> MSDNRRRRREEDDSDSENELPPSSPQQHFRGGMNPVSSPIGSPDMINPEGDDNEVDDVPDIDEVEEQMNEVDLMDDNMYEDYAADHNRDRYDPDQVDDREQQELSLSERRRIDAQLNERDRLLRNVAYIDDEDEEQEGAAQLDEMGLPVQRRRRRRQYEDLENSDDDLLSDMDIDPLREELTLESLSNVKANSYSEWITQPNVSRTIARELKSFLLEYTDETGRSVYGARIRTLGEMNSESLEVNYRHLAESKAILALFLAKCPEEMLKIFDLVAMEATELHYPDYARIHSEIHVRISDFPTIYSLRELRESNLSSLVRVTGVVTRRTGVFPQLKYVKFNCLKCGSILGPFFQDSNEEIRISFCTNCKSKGPFRVNGEKTVYRNYQRVTLQEAPGTVPPGRLPRHREVILLADLVDVSKPGEEVEVTGIYKNNYDGNLNAKNGFPVFATIIEANSIKRREGNTANEGEEGLDVFSWTEEEEREFRKISRDRGIIDKIISSMAPSIYGHRDIKTAVACSLFGGVPKNVNGKHSIRGDINVLLLGDPGTAKSQILKYVEKTAHRAVFATGQGASAVGLTASVRKDPITKEWTLEGGALVLADKGVCLIDEFDKMNDQDRTSIHEAMEQQSISISKAGIVTTLQARCSIIAAANPNGGRYNSTLPLAQNVSLTEPILSRFDILCVVRDLVDEEADERLATFVVDSHVRSHPENDEDREGEELKNNGESAIEQGEDEINEQLNARQRRLQRQRKKEEEISPIPQELLMKYIHYARTKIYPKLHQMDMDKVSRVYADLRRESISTGSFPITVRHLESILRIAESFAKMRLSEFVSSYDLDRAIKVVVDSFVDAQKVSVRRQLRRSFAIYTLGH;> MEGSTGFDGDATTFFAPDAVFGDRVRRFQEFLDTFTSYRDSVRSIQVYNSNNAANYNDDQDDADERDLLGDDDGDDLEKEKKAASSTSLNILPHRIIISLDDLREFDRSFWSGILVEPAYFIPPAEKALTDLADSMDDVPHPNASAVSSRHPWKLSFKGSFGAHALSPRTLTAQHLNKLVSVEGIVTKTSLVRPKLIRSVHYAAKTGRFHYRDYTDATTTLTTRIPTPAIYPTEDTEGNKLTTEYGYSTFIDHQRITVQEMPEMAPAGQLPRSIDVILDDDLVDKTKPGDRVNVVGVFKSLGAGGMNQSNSNTLIGFKTLILGNTVYPLHARSTGVAARQMLTDFDIRNINKLSKKKDIFDILSQSLAPSIYGHDHIKKAILLMLMGGVEKNLENGSHLRGDINILMVGDPSTAKSQLLRFVLNTASLAIATTGRGSSGVGLTAAVTTDRETGERRLEAGAMVLADRGVVCIDEFDKMTDVDRVAIHEVMEQQTVTIAKAGIHTTLNARCSVIAAANPVFGQYDVNRDPHQNIALPDSLLSRFDLLFVVTDDINEIRDRSISEHVLRTHRYLPPGYLEGEPVRERLNLSLAVGEDADINPEEHSNSGAGVENEGEDDEDHVFEKFNPLLQAGAKLAKNKGNYNGTEIPKLVTIPFLRKYVQYAKERVIPQLTQEAINVIVKNYTDLRNDDNTKKSPITARTLETLIRLATAHAKVRLSKTVNKVDAKVAANLLRFALLGEDIGNDIDEEESEYEEALSKRSPQKSPKKRQRVRQPASNSGSPIKSTPRRSTASSVNATPSSARRILRFQDDEQNAGEDDNDIMSPLPADEEAELQRRLQLGLRVSPRRREHLHAPEEGSSGPLTEVGTPRLPNVSSAGQDDEQQQSVISFDNVEPGTISTGRLSLISGIIARLMQTEIFEEESYPVASLFERINEELPEEEKFSAQEYLAGLKIMSDRNNLMVADDKVWRV;> MSQQSSSPTKEDNNSSSPVVPNPDSVPPQLSSPALFYSSSSSQGDIYGRNNSQNLSQGEGNIRAAIGSSPLNFPSSSQRQNSDVFQSQGRQGRIRSSASASGRSRYHSDLRSDRALPTSSSSLGRNGQNRVHMRRNDIHTSDLSSPRRIVDFDTRSGVNTLDTSSSSAPPSEASEPLRIIWGTNVSIQECTTNFRNFLMSFKYKFRKILDEREEFINNTTDEELYYIKQLNEMRELGTSNLNLDARNLLAYKQTEDLYHQLLNYPQEVISIMDQTIKDCMVSLIVDNNLDYDLDEIETKFYKVRPYNVGSCKGMRELNPNDIDKLINLKGLVLRSTPVIPDMKVAFFKCNVCDHTMAVEIDRGVIQEPARCERIDCNEPNSMSLIHNRCSFADKQVIKLQETPDFVPDGQTPHSISLCVYDELVDSCRAGDRIEVTGTFRSIPIRANSRQRVLKSLYKTYVDVVHVKKVSDKRLDVDTSTIEQELMQNKVDHNEVEEVRQITDQDLAKIREVAAREDLYSLLARSIAPSIYELEDVKKGILLQLFGGTNKTFTKGGRYRGDINILLCGDPSTSKSQILQYVHKITPRGVYTSGKGSSAVGLTAYITRDVDTKQLVLESGALVLSDGGVCCIDEFDKMSDSTRSVLHEVMEQQTISIAKAGIITTLNARSSILASANPIGSRYNPNLPVTENIDLPPPLLSRFDLVYLVLDKVDEKNDRELAKHLTNLYLEDKPEHISQDDVLPVEFLTMYISYAKEHIHPIITEAAKTELVRAYVGMRKMGDDSRSDEKRITATTRQLESMIRLAEAHAKMKLKNVVELEDVQEAVRLIRSAIKDYATDPKTGKIDMNLVQTGKSVIQRKLQEDLSREIMNVLKDQASDSMSFNELIKQINEHSQDRVESSDIQEALSRLQQEDKVIVLGEGVRRSVRLNNRV;> MSFDRPEIYSAPVLQGESPNDDDNTEIIKSFKNFILEFRLDSQFIYRDQLRNNILVKNYSLTVNMEHLIGYNEDIYKKLSDEPSDIIPLFETAITQVAKRISILSRAQSANNNDKDPENTSMDTDSLLLNSLPTFQLILNSNANQIPLRDLDSEHVSKIVRLSGIIISTSVLSSRATYLSIMCRNCRHTTSITINNFNSITGNTVSLPRSCLSTIESESSMANESNIGDESTKKNCGPDPYIIIHESSKFIDQQFLKLQEIPELVPVGEMPRNLTMTCDRYLTNKVIPGTRVTIVGIYSIYNSKNGAGSGRSGGGNGGSGVAIRTPYIKILGIQSDVETSSIWNSVTMFTEEEEEEFLQLSRNPKLYEILTNSIAPSIFGNEDIKKAIVCLLMGGSKKILPDGMRLRGDINVLLLGDPGTAKSQLLKFVEKVSPIAVYTSGKGSSAAGLTASVQRDPMTREFYLEGGAMVLADGGVVCIDEFDKMRDEDRVAIHEAMEQQTISIAKAGITTVLNSRTSVLAAANPIYGRYDDLKSPGDNIDFQTTILSRFDMIFIVKDDHNEERDISIANHVINIHTGNANAMQNQQEENGSEISIEKMKRYITYCRLKCAPRLSPQAAEKLSSNFVTIRKQLLINELESTERSSIPITIRQLEAIIRITESLAKLELSPIAQERHVDEAIRLFQASTMDAASQDPIGGLNQASGTSLSEIRRFEQELKRRLPIGWSTSYQTLRREFVDTHRFSQLALDKALYALEKHETIQLRHQGQNIYRSGV;> MSSPFPADTPSSNRPSNSSPPPSSIGAGFGSSSGLDSQIGSRLHFPSSSQPHVSNSQTGPFVNDSTQFSSQRLQTDGSATNDMEGNEPARSFKSRALNHVKKVDDVTGEKVREAFEQFLEDFSVQSTDTGEVEKVYRAQIEFMKIYDLNTIYIDYQHLSMRENGALAMAISEQYYRFLPFLQKGLRRVVRKYAPELLNTSDSLKRSEGDEGQADEDEQQDDDMNGSSLPRDSGSSAAPGNGTSAMATRSITTSTSPEQTERVFQISFFNLPTVHRIRDIRSEKIGSLLSISGTVTRTSEVRPELYKASFTCDMCRAIVDNVEQSFKYTEPTFCPNPSCENRAFWTLNVTRSRFLDWQKVRIQENANEIPTGSMPRTLDVILRGDSVERAKPGDRCKFTGVEIVVPDVTQLGLPGVKPSSTLDTRGISKTTEGLNSGVTGLRSLGVRDLTYKISFLACHVISIGSNIGASSPDANSNNRETELQMAANLQANNVYQDNERDQEVFLNSLSSDEINELKEMVKDEHIYDKLVRSIAPAVFGHEAVKKGILLQMLGGVHKSTVEGIKLRGDINICVVGDPSTSKSQFLKYVVGFAPRSVYTSGKASSAAGLTAAVVRDEEGGDYTIEAGALMLADNGICCIDEFDKMDISDQVAIHEAMEQQTISIAKAGIHATLNARTSILAAANPVGGRYNRKLSLRGNLNMTAPIMSRFDLFFVILDDCNEKIDTELASHIVDLHMKRDEAIEPPFSAEQLRRYIKYARTFKPILTKEARSYLVEKYKELRKDDAQGFSRSSYRITVRQLESMIRLSEAIARANCVDEITPSFIAEAYDLLRQSIIRVDVDDVEMDEEFDNIESQSHAASGNNDDNDDGTGSGVITSEPPADIEEGQSEATARPGTSEKKKTTVTYDKYVSMMNMIVRKIAEVDREGAEELTAVDIVDWYLLQKENDLGSLAEYWEERRLAFKVIKRLVKDRILMEIHGTRHNLRDLENEENENNKTVYVIHPNCEVLDQLEPQDSS;> MSAALPSIQLPVDYNNLFNEITDFLVTFKQDTLSSDATRNENEDENLDAENIEQHLLEKGPKYMAMLQKVANRELNSVIIDLDDILQYQNEKFLQGTQADDLVSAIQQNANHFTELFCRAIDNNMPLPTKEIDYKDDVLDVILNQRRLRNERMLSDRTNEIRSENLMDTTMDPPSSMNDALREVVEDETELFPPNLTRRYFLYFKPLSQNCARRYRKKAISSKPLSVRQIKGDFLGQLITVRGIITRVSDVKPAVEVIAYTCDQCGYEVFQEVNSRTFTPLSECTSEECSQNQTKGQLFMSTRASKFSAFQECKIQELSQQVPVGHIPRSLNIHVNGTLVRSLSPGDIVDVTGIFLPAPYTGFKALKAGLLTETYLEAQFVRQHKKKFASFSLTSDVEERVMELITSGDVYNRLAKSIAPEIYGNLDVKKALLLLLVGGVDKRVGDGMKIRGDINVCLMGDPGVAKSQLLKAICKISPRGVYTTGKGSSGVGLTAAVMKDPVTDEMILEGGALVLADNGICCIDEFDKMDESDRTAIHEVMEQQTISISKAGINTTLNARTSILAAANPLYGRYNPRLSPLDNINLPAALLSRFDILFLMLDIPSRDDDEKLAEHVTYVHMHNKQPDLDFTPVEPSKMREYIAYAKTKRPVMSEAVNDYVVQAYIRLRQDSKREMDSKFSFGQATPRTLLGIIRLSQALAKLRLADMVDIDDVEEALRLVRVSKESLYQETNKSKEDESPTTKIFTIIKKMLQETGKNTLSYENIVKTVRLRGFTMLQLSNCIQEYSYLNVWHLINEGNT;> MSGTANSRRKEVLRVPVIDLNRVSDEEQLLPVVRAILLQHDTFLLKNYANKAVLDALLAGLTTKDLPDTSQGFDANFTGTLPLEDDVWLEQYIFDTDPQLRFDRKCRNESLCSIYSRLFKLGLFFAQLCVKSVVSSAELQDCISTSHYATKLTRYFNDNGSTHDGADAGATVLPTGDDFQYLFERDYVTFLPTGVLTIFPCAKAIRYKPSTMATTDNSWVSIDEPDCLLFHTGTLLARWSQGMHTTSPLQIDPRANIVSLTIWPPLTTPISSKGEGTIANHLLEQQIKAFPKVAQQYYPRELSILRLQDAMKFVKELFTVCETVLSLNALSRSTGVPPELHVLLPQISSMMKRKIVQDDILKLLTIWSDAYVVELNSRGELTMNLPKRDNLTTLTNKSRTLAFVERAESWYQQVIASKDEIMTDVPAFKINKRRSSSNSKTVLSSKVQTKSSNANALNNSRYLANSKENFMYKEKMPDSQANLMDRLRERERRSAALLSQRQKRYQQFLAMKMTQVFDILFSLTRGQPYTETYLSSLIVDSLQDSNNPIGTKEASEILAGLQGILPMDISVHQVDGGLKVYRWNSLDKNRFSKLLQIHKSKQQD;> MSAIPITPTKRIRRNLFDDAPATPPRPLKRKKLQFTDVTPESSPEKLQFGSQSIFLRTKALLQKSSELVNLNSSDGALPARTAEYEQVMNFLAKAISEHRSDSLYITGPPGTGKTAQLDMIIRQKFQSLPLSLSTPRSKDVLRHTNPNLQNLSWFELPDGRLESVAVTSINCISLGEPSSIFQKIFDSFQDLNGPTLQIKNMQHLQKFLEPYHKKTTFVVVLDEMDRLLHANTSETQSVRTILELFLLAKLPTVSFVLIGMANSLDMKDRFLSRLNLDRGLLPQTIVFQPYTAEQMYEIVIQKMSSLPTIIFQPMAIKFAAKKCAGNTGDLRKLFDVLRGSIEIYELEKRFLLSPTRGSLNSAQVPLTPTTSPVKKSYPEPQGKIGLNYIAKVFSKFVNNNSTRTRIAKLNIQQKLILCTIIQSLKLNSDATIDESFDHYIKAITKTDTLAPLQRNEFLEICTILETCGLVSIKKTKCKGKTKRFVDKIDVDLDMREFYDEMTKISILKPFLH;> MAKTLKDLQGWEIITTDEQGNIIDGGQKRLRRRGAKTEHYLKRSSDGIKLGRGDSVVMHNEAAGTYSVYMIQELRLNTLNNVVELWALTYLRWFEVNPLAHYRQFNPDANILNRPLNYYNKLFSETANKNELYLTAELAELQLFNFIRVANVMDGSKWEVLKGNVDPERDFTVRYICEPTGEKFVDINIEDVKAYIKKVEPREAQEYLKDLTLPSKKKEIKRGPQKKDKATQTAQISDAETRATDITDNEDGNEDESSDYESPSDIDVSEDMDSGEISADELEEEEDEEEDEDEEEKEARHTNSPRKRGRKIKLGKDDIDASVQPPPKKRGRKPKDPSKPRQMLLISSCRANNTPVIRKFTKKNVARAKKKYTPFSKRFKSIAAIPDLTSLPEFYGNSSELMASRFENKLKTTQKHQIVETIFSKVKKQLNSSYVKEEILKSANFQDYLPARENEFASIYLSAYSAIESDSATTIYVAGTPGVGKTLTVREVVKELLSSSAQREIPDFLYVEINGLKMVKPTDCYETLWNKVSGERLTWAASMESLEFYFKRVPKNKKKTIVVLLDELDAMVTKSQDIMYNFFNWTTYENAKLIVIAVANTMDLPERQLGNKITSRIGFTRIMFTGYTHEELKNIIDLRLKGLNDSFFYVDTKTGNAILIDAAGNDTTVKQTLPEDVRKVRLRMSADAIEIASRKVASVSGDARRALKVCKRAAEIAEKHYMAKHGYGYDGKTVIEDENEEQIYDDEDKDLIESNKAKDDNDDDDDNDGVQTVHITHVMKALNETLNSHVITFMTRLSFTAKLFIYALLNLMKKNGSQEQELGDIVDEIKLLIEVNGSNKFVMEIAKTLFQQGSDNISEQLRIISWDFVLNQLLDAGILFKQTMKNDRICCVKLNISVEEAKRAMNEDETLRN;> MLNGEDFVEHNDILSSPAKSRNVTPKRVDPHGERQLRRIHSSKKNLLERISLVGNERKNTSPDPALKPKTPSKAPRKRGRPRKIQEELTDRIKKDEKDTISSKKKRKLDKDTSGNVNEESKTSNNKQVMEKTGIKEKRERE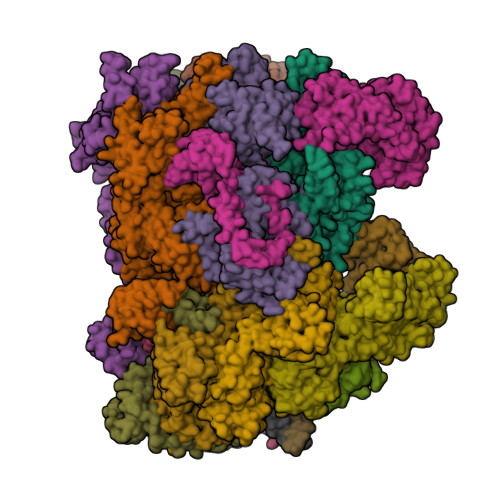KIQVATTTYEDNVTPQTDDNFVSNSPEPPEPATPSKKSLTTNHDFTSPLKQIIMNNLKEYKDSTSPGKLTLSRNFTPTPVPKNKKLYQTSETKSASSFLDTFEGYFDQRKIVRTNAKSRHTMSMAPDVTREEFSLVSNFFNENFQKRPRQKLFEIQKKMFPQYWFELTQGFSLLFYGVGSKRNFLEEFAIDYLSPKIAYSQLAYENELQQNKPVNSIPCLILNGYNPSCNYRDVFKEITDLLVPAELTRSETKYWGNHVILQIQKMIDFYKNQPLDIKLILVVHNLDGPSIRKNTFQTMLSFLSVIRQIAIVASTDHIYAPLLWDNMKAQNYNFVFHDISNFEPSTVESTFQDVMKMGKSDTSSGAEGAKYVLQSLTVNSKKMYKLLIETQMQNMGNLSANTGPKRGTQRTGVELKLFNHLCAADFIASNEIALRSMLREFIEHKMANITKNNSGMEIIWVPYTYAELEKLLKTVLNTL;> MSDLNQSKKMNVSEFADAQRSHYTVYPSLPQSNKNDKHIPFVKLLSGKESEVNVEKRWELYHQLHSHFHDQVDHIIDNIEADLKAEISDLLYSETTQKRRCFNTIFLLGSDSTTKIELKDESSRYNVLIELTPKESPNVRMMLRRSMYKLYSAADAEEHPTIKYEDINDEDGDFTEQNNDVSYDLSLVENFKRLFGKDLAMVFNFKDVDSINFNTLDNFIILLKSAFKYDHVKISLIFNINTNLSNIEKNLRQSTIRLLKRNYHKLDVSSNKGFKYGNQIFQSFLDTVDGKLNLSDRFVEFILSKMANNTNHNLQLLTKMLDYSLMSYFFQNAFSVFIDPVNVDFLNDDYLKILSRCPTFMFFVEGLIKQHAPADEILSLLTNKNRGLEEFFVEFLVRENPINGHAKFVARFLEEELNITNFNLIELYHNLLIGKLDSYLDRWSACKEYKDRLHFEPIDTIFQELFTLDNRSGLLTQSIFPSYKSNIEDNLLSWEQVLPSLDKENYDTLSGDLDKIMAPVLGQLFKLYREANMTINIYDFYIAFRETLPKEEILNFIRKDPSNTKLLELAETPDAFDKVALILFMQAIFAFENMGLIKFQSTKSYDLVEKCVWRGI;> MTISEARLSPQVNLLPIKRHSNEEVEETAAILKKRTIDNEKCKDSDPGFGSLQRRLLQQLYGTLPTDEKIIFTYLQDCQQEIDRIIKQSIIQKESHSVILVGPRQSYKTYLLDYELSLLQQSYKEQFITIRLNGFIHSEQTAINGIATQLEQQLQKIHGSEEKIDDTSLETISSGSLTEVFEKILLLLDSTTKTRNEDSGEVDRESITKITVVFIFDEIDTFAGPVRQTLLYNLFDMVEHSRVPVCIFGCTTKLNILEYLEKRVKSRFSQRVIYMPQIQNLDDMVDAVRNLLTVRSEISPWVSQWNETLEKELSDPRSNLNRHIRMNFETFRSLPTLKNSIIPLVATSKNFGSLCTAIKSCSFLDIYNKNQLSNNLTGRLQSLSDLELAILISAARVALRAKDGSFNFNLAYAEYEKMIKAINSRIPTVAPTTNVGTGQSTFSIDNTIKLWLKKDVKNVWENLVQLDFFTEKSAVGLRDNATAAFYASNYQFQGTMIPFDLRSYQMQIILQELRRIIPKSNMYYSWTQL;> MNVTTPEVAFREYQTNCLASYISADPDITPSNLILQGYSGTGKTYTLKKYFNANPNLHAVWLEPVELVSWKPLLQAIARTVQYKLKTLYPNIPTTDYDPLQVEEPFLLVKTLHNIFVQYESLQEKTCLFLILDGFDSLQDLDAALFNKYIKLNELLPKDSKINIKFIYTMLETSFLQRYSTHCIPTVMFPRYNVDEVSTILVMSRCGELMEDSCLRKRIIEEQITDCTDDQFQNVAANFIHLIVQAFHSYTGNDIFALNDLIDFKWPKYVSRITKENIFEPLALYKSAIKLFLSTDDNLSENGQGESAITTNRDDLENSQTYDLSIISKYLLIASYICSYLEPRYDASIFSRKTRIIQGRAAYGRRKKKEVNPRYLQPSLFAIERLLAIFQAIFPIQGKAESGSLSALREESLMKANIEVFQNLSELHTLKLIATTMNKNIDYLSPKVRWKVNVPWEIIKEISESVHFNISDYFSDIHE;> MSMQQVQHCVAEVLRLDPQEKPDWSSGYLKKLTNATSILYNTSLNKVMLKQDEEVARCHICAYIASQKMNEKHMPDLCYYIDSIPLEPKKAKHLMNLFRQSLSNSSPMKQFAWTPSPKKNKRSPVKNGGRFTSSDPKELRNQLFGTPTKVRKSQNNDSFVIPELPPMQTNESPSITRRKLAFEEDEDEDEEEPGNDGLSLKSHSNKSITGTRNVDSDEYENHESDPTSEEEPLGVQESRSGRTKQNKAVGKPQSELKTAKALRKRGRIPNSLLVKKYCKMTTEEIIRLCNDFELPREVAYKIVDEYNINASRLVCPWQLVCGLVLNCTFIVFNERRRKDPRIDHFIVSKMCSLMLTSKVDDVIECVKLVKELIIGEKWFRDLQIRYDDFDGIRYDEIIFRKLGSMLQTTNILVTDDQYNIWKKRIEMDLALTEPL5,5-DIFLUOROMETHYL 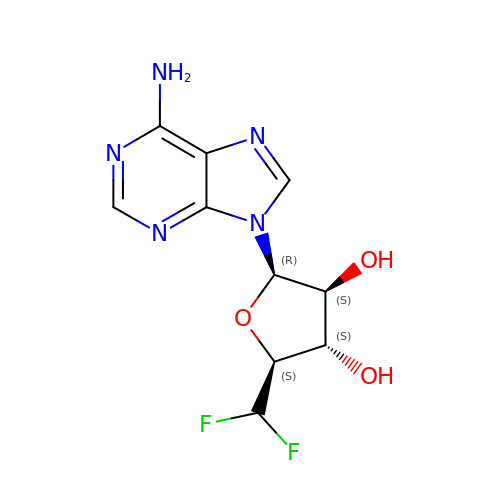ADENOSINE | C10 H11 F2 N5 O3 | YQLJSFYLQCBEKY-AVGUDYQDSA-N> SMTQNCVAPVAIIGMACRLPGAINSPQQLWEALLRGDDFVTEIPTGRWDAEEYYDPEPGVPGRSVSKWGAFLDDPAAFDPEFFGITEREAAAIDPQHRLLLETAWEAVEHSGLNPAGLAGSATGVFMGLTHNDYAHLAADAKALEGPYGFTGTSFSLASGRIAYALGVHGPAITVDTACSSSLSAIHMACRSLHDGESDVALAGGVSVLLEPRKAAGGSAAGMLSPTGHCHAFDTAADGFVSAEGCVVLTLKRLDDAVADGDRILAVIRGTATNQDGRTVNIATPSADAQAKVYRMALKAAGVEPGTVGLVEAHGTGTPVGDPLEFSSLAEVYGTDGPCALGSIKTNFGHTQSAAGALGVMKAVLALQHNVIPQNLHFTRLPDQMAEIETGLFVPETITPWPVREGQPRRAAVSAYGLSGTNVHAVLEQAPESPAETAAEAISPKAGNALVFPVSASSADALRSTAQHLADWLLRSGDGNGRGPAIDLGDLAYTLARRRGFRAARSAVLAGDRGTLVEGLRQIADGEAMPQQAVTNDDRGPVWVFSGQGSQWASMGAELLDREPAFAAAIAELEPLIAAESDFSVTEALTASE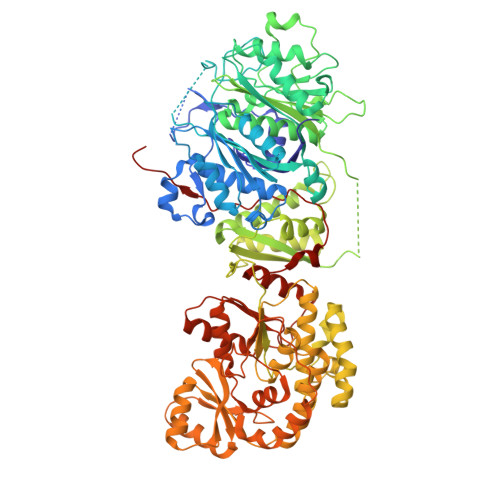TVTGIDRVQPTIFAVQVALAAAMRSHGVVPGAVIGHSMGEVAASVVSGALSLEDGVKVICRRTRLMTRIAGSGAMAMVELPAQQVLSELASRGVDDVVLSVVASPQSTVVGGATASVRELIEMWESRGVMAREIAVDVASHSPQVDPILDDLIEALADLDPAEPEIPYYSATLYDPRDYADYDAYYWADNLRHTVRFSAAVQAALEDGHRVFAELSPHPLLTHPVEQTARSLDMPLAVFAAMRRQQEMPHGLLGFVADLHSAGAAVDFSVLYPTGRLLDAPLPAWTHSTLLLDRELESSA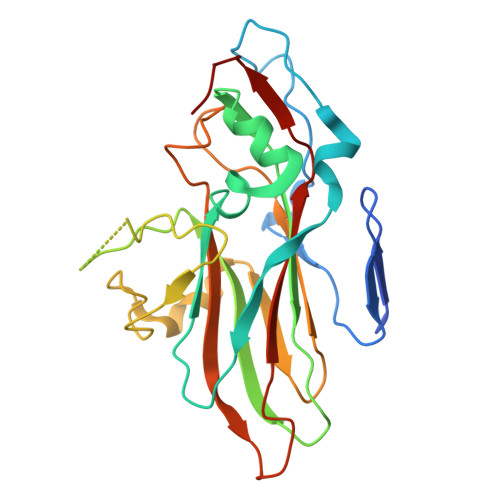> SPSAEACGYSDRVAQLTIGNSTITTQEAANIVIAYGEWPEYCPDTDATAVDKPTRPDVSVNRFFTLDTKSWAKDSKGWYWKFPDVLTEVGVFGQNAQFHYLYRSGFCVHVQCNASKFHQGALLVAVLPEYVLGTIAGGTGNENSHPPYATTQPGQVGAVLTHPYVLDAGIPLSQLTVCPHQWINLRTNNCATIIVPYMNTVPFDSALNHCNFGLLVIPVVPLDFNAGATSEIPITVTIAPMCAEFAGLRQAVKQ>NAMMYFISDTHFYHENIINLNPEVRFKGFEIVILTNLLKVLKPEDTLYHLGDFTWHFNDKNEYLRIWKALPGRKILVMGNHDKDKESLKEYFDEIYDFYKIIEHKGKRILLSHYPAKDPITERYPDRQEMVREIYFKENCDLLIHGHVHWNREGIKCACKDYRIECINANVEWNDYKPISEREIDKLISYE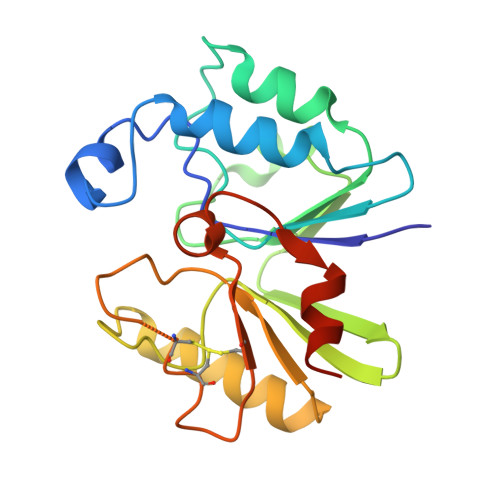KAKN[2x]GIPC1 (GAIP interacting protein, C-terminus 1) and its two paralogs GIPC2 and GIPC3 are universal adaptor proteins that bind and regulate vesicular trafficking of many transmembrane proteins. GIPCs contribute to the endocytosis process by tethering the cargo proteins on endocytic vesicles to the motor protein myosin VI. GIPCs contain a central PDZ (PSD-95, Dlg and ZO-1) domain that mediates the interaction with the C-terminal PDZ-binding motif (PBM) in cargo proteins. The transmembrane receptor PlexinD1 contains a C-terminal ‘SEA’ motif that constitutes a PBM and interacts with GIPC1.

We crystallized the GH1-PDZ-GH2 domains of mouse GIPC1 and determined its X-ray crystal structure to 1.9 Å resolution. The GH1 domain adopts an ubiquitin-like fold composed of four β-strands and one α-helix, although it lacks obvious sequence similarity to ubiquitin. A prominent feature of the GIPC1 structure is that two molecules in the asymmetric unit form a domain-swapped dimer. The domain swap is the result of an exchange of the last β-strand between the two GH1 domains. Due to the domain swap, the PDZ domain from one molecule is located in close proximity to the GH1 domain of the dimer partner. The overall shape of the dimeric GH1-PDZ module resembles a canoe with the two GH1 domains at the middle and the two PDZ domains curving upwards at each end. The GH2 domain wedges itself between the PDZ-GH2 linker and the PDZ domain, reminiscent of a passenger sitting in the canoe formed by the dimeric GH1-PDZ modules. Notably, the loop between helices α1 and α2 in the GH2 domain partially occupies the PBM-binding groove in the PDZ domain. Conversely, the PDZ domain blocks one face on the GH2 domain that binds myosin VI (as defined by the structures of the GH2/myosin VI complexes below). Therefore, the apo-GIPC1 structure represents the state in which the PDZ and GH2 domains mutually inhibit each other.

>[2x]GPHMAALRPRLVFHTQLAHGSPTGRIEGFTNVKELYGKIAEAFRLPAAEVMFCTLNTHKVDMDKLLGGQIGLEDFIFAHVKGQRKEVEVFKSEEALGLTITDNGAGYAFIKRIKEGSVIDHIQLISVGDMIEAINGQSLLGCRHYEVARLLKELPRGRTFTLKLTEPRKAFDMISQRSAGGHPGSGPQLGTGRGTLRLRSRGPATVEDLPSAFEEKAIEKVDDLLESYMGIRDTELAATMVELGKDKRNPDELAEALDERLGDFAFPDEFVFDVWGAIGD>MSTPQDNANTVHRYLEFVAKGQPDEIAALYADDATVEDPVGSEVHIGRQAIRGFYGNLENVQSRTEVKTLRALGHEVAFYWTLSIGGDEGGMT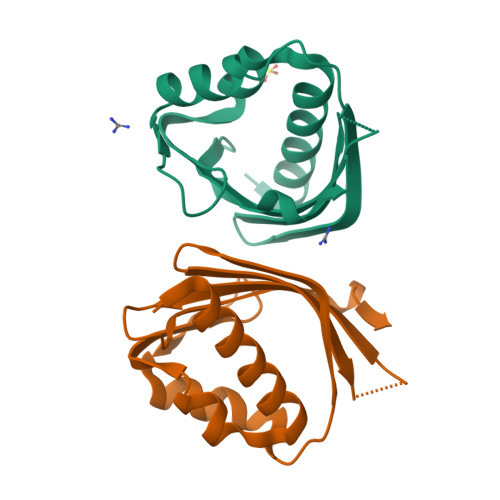MDIISVMTFNDDGRIKSMKAYWTPENITQR[2x]> MLSKVTRRFLNYNQIYCFASQHGAEHHKLTASDEAYLNEVRQRYVTPDMEKWAYLDYKKHPSTTLSHYDHKSKDYVESERDDYNADVATNSHNKLIDDFKRNLQMQRKVHDILQKMDRPYLRGVPGVTKNISAGLQDYSAPVSKKSQSDPNDFYRDAYRNENRWIDQSVFTPKTSKMTHYDVEWPKELASRPVTKKFHHDKGYKYDVTTPYDQRYNYVADRLGHPEILGNPFERLMRLEGDIYHPNYLDQPFVKVPNANPNASLNFEEGEVLYENTRLLEWAKFWNYSVVVGYLWCAYFVPYNIFFKTHMPLEHAYDNLFFPYFQHTHFLWDNNALHIPTVGGVAIYATYIALSYINNIWKDYVVRAQFSKDKELLFVTRVSPFGTTEEEVYEVAHLEHLPPSVRSGVKDLSAQDADGLVDVTCMSSQRSLVFY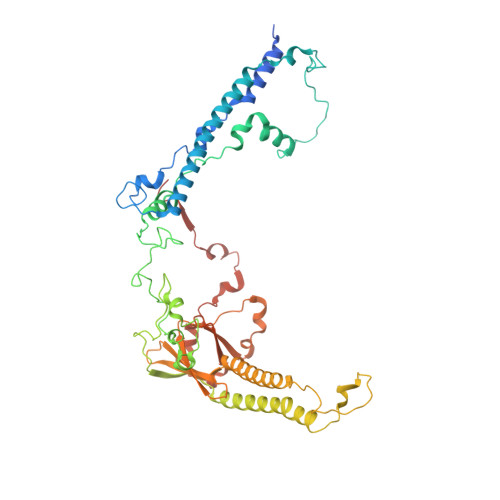KGDQYWNPKVYNDFINQTSNLWTRNYTGYNRLEVQNSVEQVKIGFSHSSQPKLEKK> MTWLTKIVPDLRYRQTRADFRTAGNLHRKLIRLSSDLGEERIANPRQQSGLLFRIEETRNELYLLVQSHSPLRVDRLGPGYHGVQMRNLDPFLARLDKGSRVRYRIVASPTKRLGRSENNTQRLGLKEPPKKPREYTWALRGAAAEEWWHSRAAANGLELLSTYAQTLDDVRDPGTADRSRKIRHPAVRFDGEAVISDVDAVRHAVLNGIGRGKSYGCGLLSLALIEEGEHG;>[2x]MNSDYILQHADALVKRVSKLIVNEPAARAALRRGVGLAPEDPRMLAAHRVVAPYVPVPTDYDVDRRRAASLWDVHAVERAFYAVAAIMAAQPRSARDQEAEATEEQTGEPQDSEALTEPTPAEESSATKDGKPDRRPNLGVSLAQAVFDKGLNADSTEQRLHLIARQNLDGVHRHLPRLVLYLRSDQVHIDWGILIRDLARWGHTPRHVAREWVQDYHRTLETLTRQAEQKNKNNTTDEEAEAA;> MLSVALCFLVGGAIPSPPSFDVTIAPWLIARSRDVLAAPEMLGLRDVLIRSHELSDVEIPLPPGAAVLWRILALITARITGLDQPPNKNPKRKWQARRSQILSKGRLDPEAVDAYFADYSERFDLFHPERPWLQDPRLREECPKTSGVNKLAWGRTAGENQVWLGGHHHDLDPHPLDSAEAVWHLLATLGYGPSGMCTARVVRGRSERNVTAGPLRGTVSYHPLGRTLFESLILNIPYPGTGAADLAFWEQPELNDPLGLPEESAGLAGILRLDHFRHAVLLHPSPDGSHVVDAWVTWAWRERNISPELDPYLIYQTSKEGRVYPRPAEAERAIWRDLDALLHYGEDGNYRPTILDNCTPLAQVPQEVLDSLRLRAFGFDQDGQARDKQWFTATTPAVLRWLADRETDDNENARIVRRI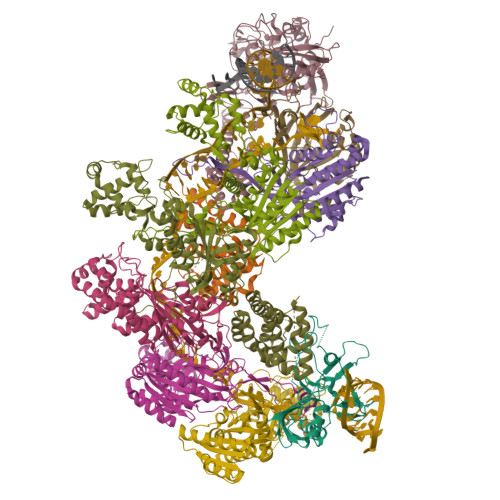TLARKAAEALGRRLEKACKEAWKESNSPSSTSSGTNAKTETGVGPWVQHGMSRYWAKAEPVFWNIVYDRPAQGYTPGMAGPGNAFNLVALAAYDEVTGPYCERPRVAKVVERHRSTLFSNWTPKQDKEAA;>MTFVDIHAIQTLPYSNINRDDLGSPKTVVYGGKERTRVSSQSWKRAVRHEVEARLGDKAVRTRRIISEIAKRLRERGWDADLADAGARQVVLSVGKKSGIKLEKEKDSEAPATSVLFYLPVPAIDELAAIADEHRDAVAKEAAKKTPKGILPADRITEVLKSRNVSVNLFGRMLAELPSTEVDGAVQFAHAFTVHGTTVEVDFFTAVDDIPKENDHGSGHMNAGQFSAGTFYRYANVNLDRLVENTGDAQTARTAVAEFLRAFLSTVPSGKQNATAAMTLPDLVHIAVRFDRPISFAPAFETALYGSDGYTLRACQELNNYAERLREVWPDDAIRGYATVENKTDLAALGERYDSYPALIDAMVAAAFEGERE[6x];> MSGFLLRLAGPMQSWGEHSMFGERDTLPYPSRSGLIGMFAAAQGVRRGDPLDRYKELKFTVRVDRPGVRLVDFHTIGGGLPKERTVPTAAGERRDPKKATIVTSRSYLADAVFTVAVTGPEADTIADALAAPYWQPYLGRRAFVPDPLLVLRRRVADPVRELVEAVPLPHRRVEEDAATVLVDLIYEEGEYPDTRTLTVLNDVPLSFDSKSRRYSTRQIRVVPTEVPATLVAGPGRDYQNKLFTYVKQCAEEAA> SNAMALDSAKKAEIVAKFAKKPGDTGSTEVQVALLTARIAELTEHLKIYKKDFSSRLGLLKLVGQRKRLLSYLKRKDYNSYSKLITELNLRD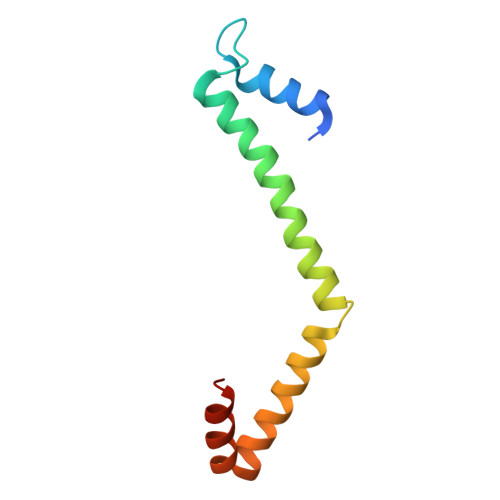K[[(2R,3S,4R,5R)-5-(6-aminopurin-9-yl)-4-oxidanyl-3-phosphonooxy-oxolan-2-yl]methoxy-oxidanyl-phosphoryl] 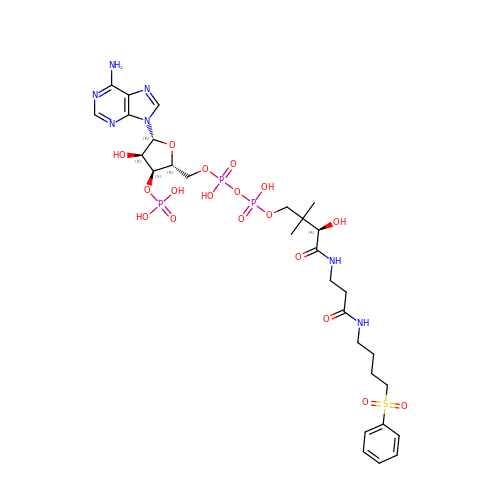[(3R)-2,2-dimethyl-3-oxidanyl-4-oxidanylidene-4-[[3-oxidanylidene-3-[4-(phenylsulfonyl)butylamino]propyl]amino]butyl] hydrogen phosphate | C29 H44 N7 O18 P3 S | VRGBEUJWLKBAGR-VXAHOBLNSA-N>MVSDYVPDAGHLVWLNFTPQAGHEQGGRRPALVLSPAAYNGVTGLMQACPVTSRAKGYPFEVTLPAHLGVSGVVLADHCRSLDWRSRRAEQLAEAPADVLAEVRGKLGSLLGMSEKA[4x];>MTSQIQKWGNSLALRIPKALAQQVGLTQSSEVELLLQDGQIVIRPVPARQYDLAALLAEMTPENLHGETDWGALEGREEW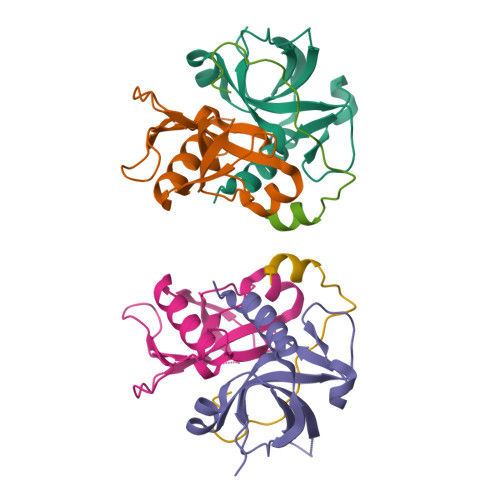[2x]>HDVTEQQKIDNDRKQFVSNVSHELRTPLTSLRSYIEALSDGAWKDPEVAPGFLKVTQEETDRMIRMINELLSLSRMDSGTTRVDMELVNINEMFNYVLDRFDMILKKDDNPAKYYTIKREFTKRDLWVEIDTDKFTQVLDNIMNNAIKYSPDGGVVTCRLLETHNQVIISISDQGLGIPRADLGHVFDRFFRVDKARSRAQGGTGLGLAISKEVVQMLGGRIWVDSVEGKGST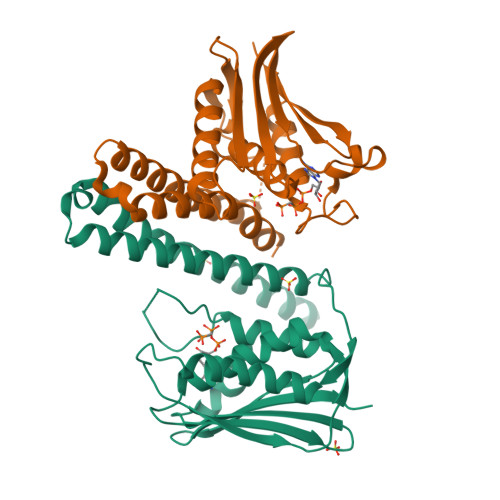FYISLPYEPYEEEDLWDDDSQA[2x]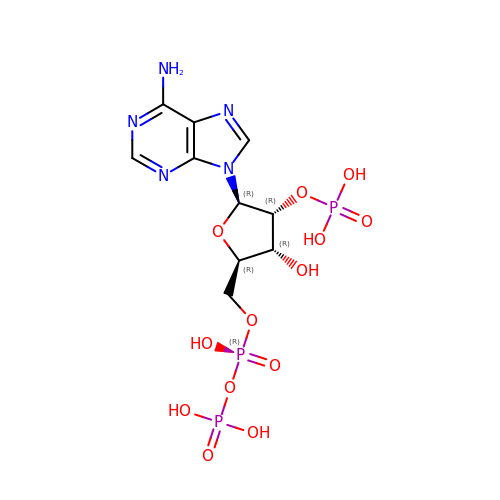2'-MONOPHOSPHOADENOSINE-5'-DIPHOSPHATE | C10 H16 N5 O13 P3 | YPTPYQSAVGGMFN-KQYNXXCUSA-N> QDTSPDTLVVTANRFEQPRSTVLAPTTVVTRQDIDRWQSTSVNDVLRRLPGVDITQNGGSGQLSSIFIRGTNASHVLVLIDGVRLNLAGVSGSADLSQFPIALVQRVEYIRGPRSAVYGSDAIGGVVNIITTRDEPGTEISAGWGSNSYQNYDVSTQQQLGDKTRVTLLGDYAHTHGYDVVAYGNTGTQAQTDNDGFLSKTLYGALEHNFTDAWSGFVRGYGYDNRTNYDAYYSPGSPLLDTRKLYSQSWDAGLRYNGELIKSQLITSYSHSKDYNYDPHYGRYDSSATLDEMKQYTVQWANNVIVGHGSIGAGVDWQKQTTTPGTGYVEDGYDQRNTGIYLTGLQQVGDFTFEGAAR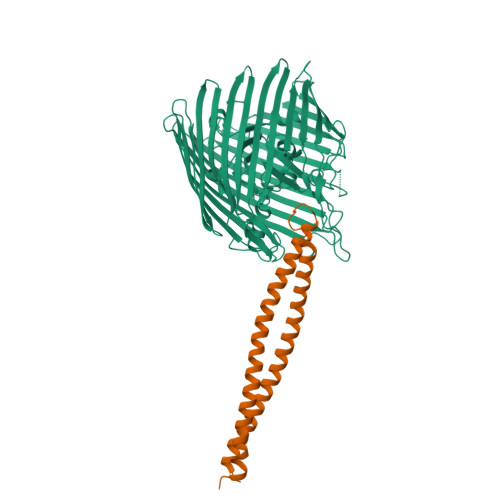SDDNSQFGRHGTWQTSAGWEFIEGYRFIASYGTSYKAPNLGQLYGFYGNPNLDPEKSKQWEGAFEGLTAGVNWRISGYRNDVSDLIDYDDHTLKYYNEGKARIKGVEATANFDTGPLTHTVSYDYVDARNAITDTPLLRRAKQQVKYQLDWQLYDFDWGITYQYLGTRYDKDYSSYPYQTVKMGGVSLWDLAVAYPVTSHLTVRGKIANLFDKDYETVYGYQTAGREYTLSGSYTF;> THPVEAAERNYERARAELNQANEDVARNQERQAKAVQVYNSRKSELDAANKTLADAIAEIKQFNRFAHDPMAGGHRMWQMAGLKAQRAQTDVNNKQAAFDAAAKEKSDADAALSAAQERRKQKENKEKDAKDKLD> MGSSHHHHHHSSGLEVLFQGPASNKVYEKTGDSVIVKVQHKETGGPRLVRLQVMGDKLIHVSATADSKFADPQSLIVVPQKKQTSFAVVQNGDTITVSTEEVKASVLASTGEVWFTDKNGELILQENKGGGKTFTPIEVEGTKGYTVCQVFESPEDEAFYGLGQHQADEFNYKGKNEELFQYNTKVSVPFVVSNKNYGILLDSYSFCRFGNPNDYSQLNRIFKLYDKTGQEGALTGTYVPKKGETLVRREDSIYFENLKTIENLPKKLPLMGAKVTYEGEIEPAQTGEFKFILYYAGYVKVYLNNEPVVPERWRTAWNPNSYKFAAHLEAGKRVPLKIEWQPDGGQSYCGLRALTPVNPEEQGKQSWWSEMTKQLDYYFMAGENMDDVISGYRSLTGKSPVMPKWAMGFWQSREKYNTQEEMLGALKGFRDRKIPLDNIVLDWNHWPENAWGSHEFDKARFPDPKAMVDSIHAMHARMMISVWPKFYVTTEHFKEFDENGWMYQQSVKDSLKDWVGPGYHYGFYDAYDPDARKLFWKQMYEHYYPLGIDAWWMDASEPNVRDCTDLEYRKALCGPTALGSSTEFFNAYALMNAEAIYDGQRGVDNNKRVFLLTRSGFAGLQRYSTATWSGDIGTRWEDMKAQISAGLNFAMSGIPYWTMDIGGFCVENRYVAGQKQWNATKTENADYKEWRELNTRWYQFGAFVPLYRAHGQYPFREIWEIAPEGHPAYQSVVYYTKLRYNMMPYIYSLAGMTWFDDYTIMRPLVMDFTADAEVNDIGDQFMFGPSFMVSPVYRYGDRSREIYFPQAEGWYDFYSGKFQAGGERKVIEAPYERIPLYVRAGAIIPFGDDIQYTDEKPAEHIRLYIYQGADGEFTLYEDEGVNYNYEQGMYAMIPMKYDEATKTLVIGERQGEFPGMLKERTFTVVTVNKEKAQPFDLNAKGVTVKYNGSEQTLKL

In this context, we recently reported the characterization of a novel xyloglucan utilization locus (XyGUL) that confers Bacteroides ovatus, and species harbouring syntenic XyGULs, with the ability to utilize this abundant vegetable polysaccharide across sampled human populations. Here, we present the three-dimensional structures of BoGH31, BoGH43A, BoGH43B and BoGH3B, expanding our knowledge of the structural determinants required for xyloglucan degradation. Our analyses highlight key adaptations in these enzymes that confer their specificity for xyloglucan oligosaccharides, while also providing a rationale for the maintenance of two divergent genes coding for GH3 enzymes, and similarly two divergent genes for GH43 family members, within the same PUL. While we were unable to determine a structure for BoGH3A, our structural and sequence analysis of BoGH3B has also allowed us to highlight further potential differences between these two enzymes encoded by the operon. Together with existing biochemical data, our analyses of the three-dimensional structures, and various enzyme-inhibitor complexes, of BoGH31, BoGH43A, BoGH43B and BoGH3B provide molecular-level insight into the stepwise breakdown of xyloglucan by the BoXyGUL.

Within XyGULs, GH31 α-xylosidases play an essential role removing xylose from the non-reducing end of processed xyloglucan oligosaccharides. Indeed, deletion of the gene encoding GH31 from the XyGUL completely abrogates the ability of B. ovatus to grow on XyG and XyGOs. Consistent with this role, the GH31 α-xylosidase present within the Bo XyGUL (BoGH31) has been shown to be highly active against native XyGO substrates (XXXG and XLLG, nomenclature according to [34]), rather than disaccharide-configured activity probes, such as Xyl-α-PNP, despite the presence of optimized chemical leaving groups requiring little protonic assistance from the enzyme. Crystals of BoGH31 were obtained by hanging drop vapour diffusion (19°C) using 0.2 M potassium thiocyanate, 14–20% (w/v) PEG-3350 as mother liquor and were used for subsequent structure determination. However, by far the closest structural match to BoGH31 was CjXyl31A (Z score = 33.1, with RMSD = 1.15 Å across 888 matched Cα positions). As observed for CjXyl31A, BoGH31 presents with an extensive, modular structure featuring several accessory domains appended to a well-conserved TIM barrel-like structure (for a full description of terms and domain nomenclature see [55]). The catalytic core of BoGH31 is composed of residues 384 to 758, which form the central (β/α)8 (TIM) barrel fold and harbour the active site (discussed below). The domains decorating the central catalytic unit include an N-terminal β-sandwich domain formed by residues 16 to 213 with additional strands contributed by residues 363 to 383 when the peptide chain returns from a PA14 domain (residues 214 to 362).> SRLNRESVIDAALELLNETGIDGLTTRKLAQKLGIEQPTLYWHVKNKRALLDALAVEILARHHDYSLPAAGESWQSFL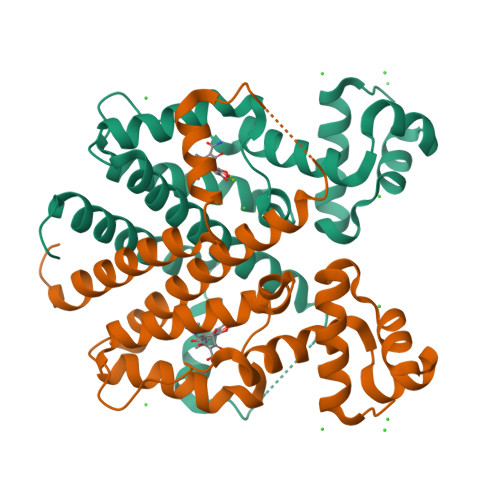RNNAMSFRRALLRYRDGAKVHLGTRPDEKQYDTVETQLRFMTENGFSLRDGLYAISAVSHFTLGAVLAQQEHTAALTDRPAAPDENLPPLLREALQIMDSDDGEQAFLHGLESLIRGFEVQLTALLQIV> MPRLIKDRVPTPERSVGERVRDFGEVNLGYSWELALREAERCLQCPVEYAPCIKGCPVHINIPGFIKALRENRDNPSKAVREALRIIWRDNTLPAITGRVCPQEEQCEGACVVGKVGDPINIGKLERFVADYAREHGIDDELLLEEIKGIKRNGKKVAIIGAGPAGLTCAADLAKMGYEVTIYEALHQPGGVLIYGIPEFRLPKEIVKKELENLRRLGVKIETNVLVGKTITFEELREEYDAIFIGTGAGTPRIYPWPGVNLNGIYSANEFLTRINLMKAYKFPEYDTPIKVGKRVAVIGGGNTAMDAARSALRLGAEVWILYRRTRKEMTAREEEIKHAEEEGVKFMFLVTPKRFIGDENGNLKAIELEKMKLGEPDESGRRRPIPTGETFIMEFDTAIIAIGQTPNKTFLETVPGLKVDEWGRIVVDENLMTSIPGVFAGGDAIRGEATVILAMGDGRKAAKAIHQYLSKEK;> MVVMVMMFKILRKERLAPGINLFEIESPRIAKHAKPGQFVMIRLHEKGERIPLTIADVDISKGSITIVAQEVGKTTRELGTYEAGDYILDVLGPLGKPSHIDYFGTVVMIGGGVGVAEIYPVAKAMKEKGNYV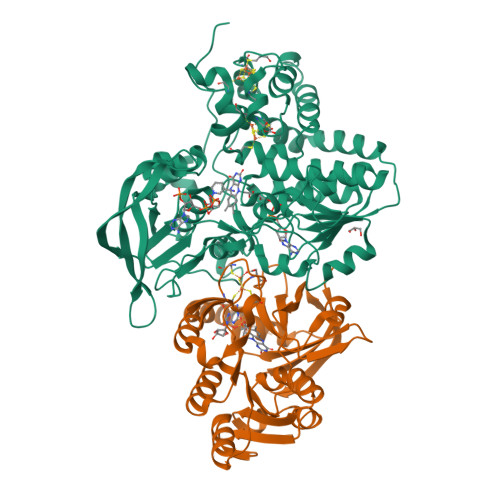ISILGFRTKDLVFWEDKLRSVSDEVIVTTNDGSYGMKGFTTHALQKLIEEGRKIDLVHAVGPAIMMKAVAELTKPYGIKTVASLNPIMVDGTGMCGACRVTVGGEVKFACVDGPEFDAHLVDWDQLMNRLAYYRDLEKISLEKWERERRMV>[2x]MEKYTIKETILTFNNEFNDPLDKYYKILSNPKIDTIEFGEKFNQEIDHLIPSNIKVIKFGWTSEFNKDVNFLTESLTEIYYGIYKNHSLEELQNLPKSLLKLKLGDVFNQEIVENVLPGGLTHLTFGEEFNQKIVENVLPGGLTHLTFGEEFNQKIVENVLPNSLTHLSFGDCFNQKITENVLPNSLTYLEFGRNFNQKITENVLPNSLTHLTFGWYFNQQITENVLPNSLTYLEFGRNFNQQITENVLPNSLTYLEFGRNFNQQITENVLPNSLTHITFGNNFNQIITENVLP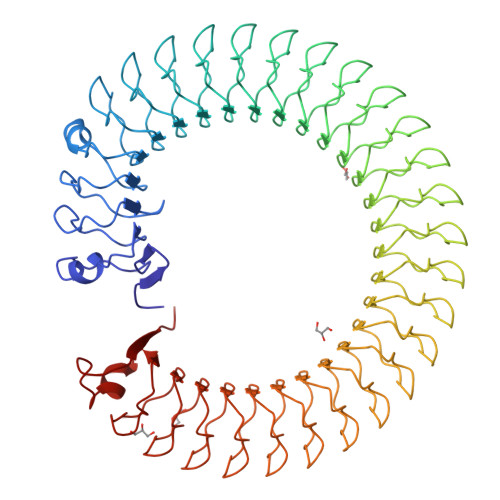NSLTHLTFGNNFNQIITENVLPNSLTHLTFGDDFNQIITENVLPNSLTHLTFGDDFNQIITENVLPNSLTHLTFGDDFNQIITENVLPNSLVHLSFGCEFNQEIAEKVLPNSLTYLELGHNFNQKIIENVLPNGLVHLSFGCKFNQEIVENVLPDSLTHLSFGHCFNQKITENVLPNSLTYLELGHNFNQKIIENVLPDRLTYLELGHDFNQKIMENVLPNSLTHLIFGTSFNQNLTENVLPNSLTHLTFGTCFNQKIIENVLPNSLTHLEFGPKFNQKITENVLPNSLTHLTFGTSFNQKITENVLPNGLTYLTFGLRFNQKITENVLPCSLTHLTFGWYFNQELTENVLPDTLKVLKIYYGNKDIILKNIDTSKIKFKIEYFNKN>[2x]SRAYDLVVIGAGSGGLEAGWNAASLHKKRVAVIDLQKHHGPPHYAALGGTCVNVG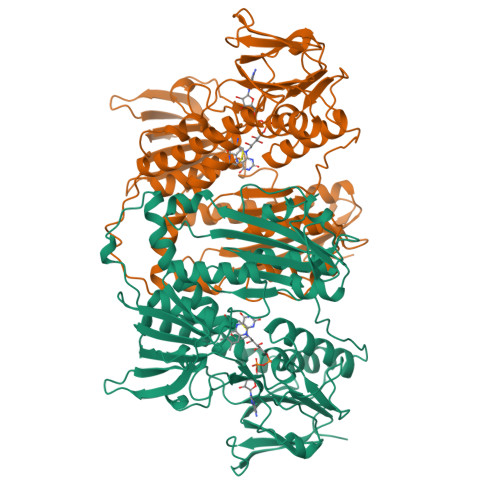CVPKKLMVTGANYMDTIRESAGFGWELDRESVRPNWKALIAAKNKAVSGINDSYEGMFADTEGLTFHQGFGALQDNHTVLVRESADPNSAVLETLDTEYILLATGSWPQHLGIEGDDLCITSNEAFYLDEAPKRALCVGGGYISIEFAGIFNAYKARGGQVDLAYRGDMILRGFDSELRKQLTEQLRANGINVRTHENPAKVTKNADGTRHVVFESGAEADYDVVMLAIGRVPRSQTLQLEKAGVEVAKNGAIKVDAYSKTNVDNIYAIGDVTDRVMLTPVAINEGAAFVDTVFANKPRATDHTKVACAVFSIPPMGVCGYVEEDAAKKYDQVAVYESSFTPLMHNISGSTYKKFMVRIVTNHADGEVLGVHMLGDSSPEIIQSVAICLKMGAKISDFYNTIGVHPTSAEELCSMRTPAYFYEKGKRVEKIDSNL> EGGQGLIEA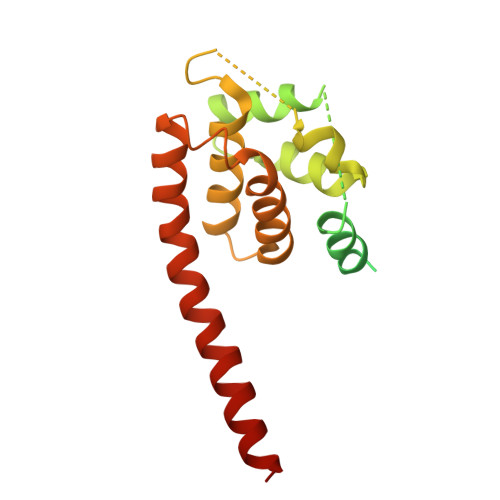ALEAEEEQAEDDGVMAPIIDQLSADMMTLSLVPRSRWQTLLHIDIIKARNKPKEPPKAPEKAPFFLPPVGQNGISSLIPQEDAKAKKEKAAANGASRITKLDLTRQEQTFTSKLLVGGAKGDYTDFIEHLKALPPAAADLELRSLSIGNGDEATNELLHFIRALTSRLVARRDYELTQAWMTVFLRLHFDLIMENEELLQALGEWREHQARERDRLSELVGYCGGVVSFLRSPRT>[8x]MNLIKEDMRVKVHMEGNVNGHAFVIEGEGKGKPYEGTQTLNLTVKEGAPLPFSYDILTTALHYGNRVFTKYPEDIPDYFKQSFPEGYSWERTMTYEDKGICTIRSDISLEGDCFFQNVRFNGMNFPPNGPVMQKKTLKWEPSTEKLHVRDGLLVGNINMALLLEGGGHYLCDFKTTYKAKKVVQLPDYHFVDHRIEILSNDSDYNKVKLYEHGVARYSPLPSQAW

The DendFP from Dendronephthya sp is a member of the Kaede-like group of photoconvertible fluorescent proteins. This FP is irreversibly converted from a green to red fluorescent state following irradiation with light from the UV region of the spectrum. The excitation/emission maxima of the green and red state of DendFP are 492/508 and 555/575 nm, respectively. The spectroscopic analysis showed that Fe2+, Fe3+, and Cu2+ significantly reduced the fluorescence emission of DendFP.

Thus, we focused on determining the native crystal structure of DendFP to investigate its metal-binding sites via comparison with those of previously reported quenchable metal-bound FPs. The DendFP crystal belongs to the orthorhombic space group P212121, with a = 115.826 Å, b = 124.737 Å, and c = 129.059 Å. The final model of DendFP was refined to a 2.60 Å resolution, with Rwork and Rfree of 23.42 and 28.13%, respectively. DendFP possesses a typical β-barrel fold, similar to other GFP-like fluorescent proteins. The chromophore of DendFP consisted of the tripeptide His62-Try63-Gly64 located inside the β-barrel and showed a nearly planar conformation with a cis-configuration. There are eight DendFP molecules in the asymmetric unit, which represent two tetrameric DendFP. In each tetrameric formation of DendFP, the two dimer molecules are related by a non-crystallographic two-fold pseudosymmetry axis perpendicular to the β-barrel. In its tetrameric formation, metal ions cannot access the interface of each molecule, which represents a site where metals cannot bind to DendFP. Following the superimposition of the crystal structures of DendFP and Dronpa, the metal-binding sites His194, His210, and His212 of Dronpa were structurally identical to Arg194, Tyr210, and His212 of DendFP, respectively. The metal-binding sites of the DendFP crystal structure were compared to those of iq-mEmerald, and Dronpa. DendFP is considered to be involved in metal binding via other types of amino acids, unlike the previously described metal-binding modes of FPs, which utilize two histidines.>MVLGKPQTDPTLEWFLSHCHIHKYPSKSTLIHQGEKAETLYYIVKGSVAVLIKDEEGKEMILSYLNQGDFIGELGLFEEGQERSAWVRAKTACEVAEISYKKFRQLIQVNPDILMRLSAQMARRLQVTSEKVGNLAFLDVTGRIAQTLLNLAKQPDAMTHPDGMQIKITRQEIGQIVGCSRETVGRILKMLEDQNLISA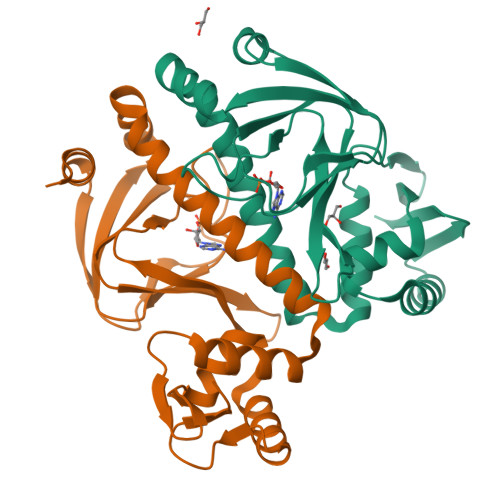HGKTIVVYGTR[2x]>GPHMEVGTVVQEEMKFRGSEFAVKVEMAERLLIVEISDVVTADQWRGEFGPAYIEDLTRKTGNFKQFPVFCSMLESAVHKSSDSVTLDLLTYSDLELLRNRKAGVVGRPRAQPQSPALSAKRYLILIYTVEEARIHYPLPLPYLGKPDPAELQKEIRALRSELKTLGLRGD[2x]

The highly conserved coiled-coil domain-containing protein 61 (CCDC61, also known as variable flagellar number 3, VFL3) is one of these understudied proteins. Here, we identify CCDC61 as a highly conserved paralog of SAS6, a key organizer of the central scaffold around which centrioles are formed (Leidel et al., 2005). Our crystal structures of CCDC61 demonstrate that it adopts a SAS6-like fold and forms oligomers through two homodimerization domains in a similar way to SAS6: an N-terminal globular head and a parallel coiled-coil domain. Further analysis of CCDC61 reveals that its coiled-coil domains are capable of directly interacting with microtubules.

To further confirm higher-order oligomer formation of zCCDC611−170 in solution, we subjected this construct, as well as its F129E/D130A mutant that disrupts the head-to-head interaction in zCCDC61, to size-exclusion chromatography with multi-angle light scattering analysis. In this experiment, the His6-lipoyl domain tag of each construct was retained to stabilize the corresponding proteins at high concentrations. The results shown in Figure 2D demonstrate that the wild-type, but not the head-to-head dimerization-deficient mutant, was able to form higher-order oligomers beyond the coiled-coil-mediated dimer.>GPLGSSTMGQVGRQLAIIGDDINRRYDSEFQTMLQHLQPTAENAYEYFTKIATSLFESGINWGRVVALLGFGYRLALHVYQHG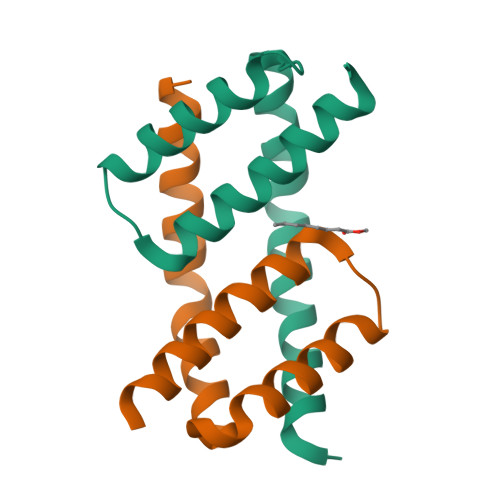LT[8x]> MNSLFNQEVQIPLTESYCGPCPKNWICYKNNCYQFFDESKNWYES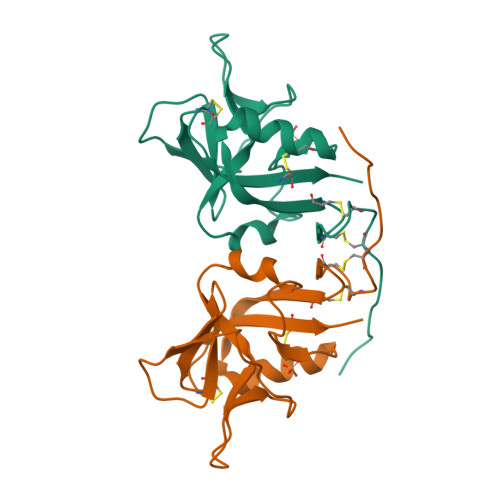QASCMSQNASLLKVYSKEDQDLLKLVKSYHWMGLVHIPTNGSWQWEDGSILSPNLLTIIEMQKGDCALYASSFKGYIENCSTPNTYICMQRTV Siastatin B is a potent and effective iminosugar inhibitor of three diverse glycosidase classes, namely, sialidases, β-d-glucuronidases, and N-acetyl-glucosaminidases. Surprisingly, siastatin B also inhibits both β-glucuronidases and human heparanase, which cleave β-glucuronic acid residues but not sialic acid or N-acetylated sugars. Herein, we show through crystallographic analysis of protein-inhibitor complexes that siastatin B generates both a hemiaminal and a 3-geminal diol iminosugar (3-GDI) that are, rather than the parent compound, directly responsible for enzyme inhibition. Notably, 3-GDIs are a new class of iminosugar glycoside hydrolase inhibitor, that have been shown to inhibit both GH2 and GH79 β-glucuronidases.

However, we were surprised to find that although each of the structures contains a ligand present with full occupancy in the active site, none of the observed ligands are siastatin B. Instead, siastatin B breakdown products are present in all structures. Three of the four enzymes (AcGH79, BpHEP, and EcGusB) contained “galacturonic-noeuromycin” bound in the −1 position of the active site, as opposed to siastatin B. The smaller functional group at the 2-position is both well accommodated within the active sites of these enzymes and the correct functional group (OH instead of NH-acetyl). The 2-hydroxyl is within hydrogen bonding distance of the catalytic nucleophile and an active site asparagine in all three of these structures, thereby mimicking the interactions seen for natural substrates28 and other inhibitors. The 4-hydroxyl of 4 has galacto-stereochemistry in contrast to the gluco-configuration of the natural enzyme substrate; however, this position also appears to have productive binding to the active site. The 4-hydroxyl of 4 forms hydrogen bond interactions with the enzyme active site, for both AcGH79 and EcGusB, see Figure 2AC. We however show here that three of the four enzymes that were soaked with siastatin B have a galacturonic acid-configured noeuromycin bound in their active site.

>SHMLRPVETPTREIKKLDGLWAFSLDRENCGIDQRWWESALQESRAIAVPGSFNDQFADADIRNYAGNVWYQREVFIPKGWAGQRIVLRFDAVTHYGKVWVNNQEVMEHQGGYTPFEADVTPYVIAGKSVRITVCVNNELNWQTIPPGMVITDENGKKKQSYFHDFFNYAGIHRSVMLYTTPNTWVDDITVVTHVAQDCNHASVDWQVVANGDVSVELRDADQQVVATGQGTSGTLQVVNPHLWQPGEGYLYELCVTAKSQTECDIYPLRVGIRSVAVKGEQFLINHKPFYFTGFGRHEDADLRGKGFDNVLMVHDHALMDWIGANSYRTSHYPYAEEMLDWADEHGIVVIDETAAVGFNLSLGIGFEAGNKPKELYSEEAVNGETQQAHLQAIKELIARDKNHPSVVMWSIANEPDTRPQGAREYFAPLAEATRKLDPTRPITCVNVMFCDAHTDTISDLFDVLCLNRYYGWYVQSGDLETAEKVLEKELLAWQEKLHQPIIITEYGVDTLAGLHSMYTDMWSEEYQCAWLDMYHRVFDRVSAVVGEQVWNFADFATSQGILRVGGNKKGIFTRDRKPKSAAFLLQKRWTGMNFGEKPQQ[2x]>MMSETAPLPSASSALEDKAASAPVVGIIMGSQSDWETMRHADALLTELEIPHETLI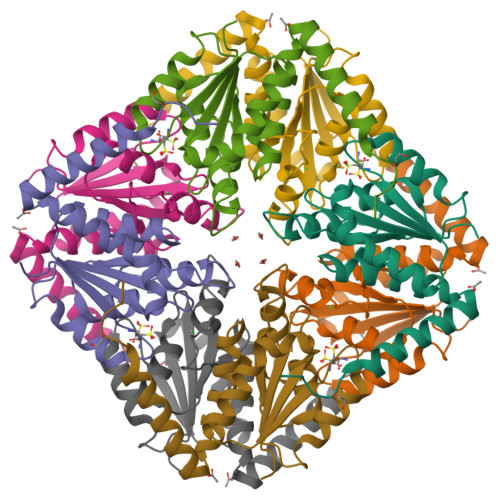VCAHRTPDRLADYARTAAERGLNVIIAGAGGAAHLPGMCAAWTRLPVLGVPVESRALKGMDSLLSIVQMPGGVPVGTLAIGASGAKNAALLAASILALYNPALAARLETWRALQTASVPNSPITEDK[2x]> MATPDQKSPNVLLQNLCCRILGKSEADVAQQFQYAVRVIGSNFAPTVERDEFLVAEKIKKELTRQRREADAALFSELHRKLHSQGVLKNKWSILYLLLSLSEDPRKQPSKVSGYAALFAQALPRDAHSTPYYYARPQSLPLNYQERGAPSAQSAGSAGSSGVSSLGTYALNGPTPPPPPPALLPGQPLPAPGVGDGLRQQLGSRLAWTLTASQPSLPSTTSKAVPSSGSRGAARPRREGDAAAGAVEVTEAALVRDILYVFQGIDGKHVKMSNADNCYTVEGKANLSKSLRDTAVRLAELGWLHNKIRKYTDQRSLDRSFGLVGQSFCAALHQELREYYRLLSVLHSQLQLEDDQGVNLGLESSLTLRRLLVWTYDPKMRLKTLAALVDHCQGRKGGELASAVHAYTKTGDPYARSLVQHILSLVSHPVLSFLYRWIYDGELEDTYHEFFVASDPAVKADRLWHDKYALRKPMIPSFMTMDQCRKVLLIGKSINFLHQVCHDQT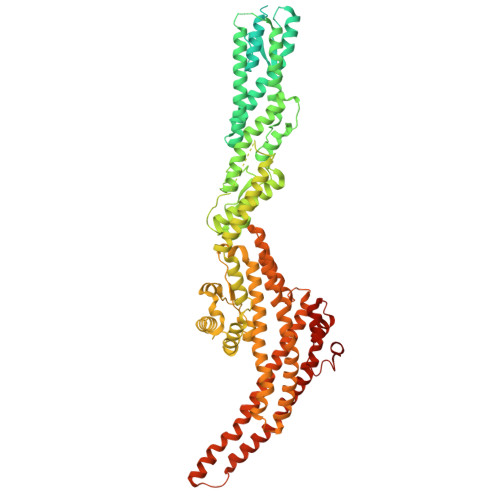PTTKMIAVTKSAESPQDAADLFTDLENAFQGKIDAAYFETSKYLLDVLNKKYSLLDHMQAMRRYLLLGQGDFIRHLMDLLKPELVRPATTLYQHNLTGILETAVRATNAQFDSPEILKRLDVRLLEVSPGDTGWDVFSLDYHVDGPIATVFTRECMSHYLRAFNFLWRAKRVEYILTDIRKGHMCNARLLRSMPEFSGVLHHCHILASEMVHFIHQMQYYVTFEVLECSWDELWNRVQRAQDLDHIIAAHEAFLGTVISRCLLDSDSRALLNQLRAVFDQIIELQNTQDAIYRAALEELQRRLQFEEKKKQREAEGQWGVSAAEEEQEKRRVQEFQESIPKMCSQLRILTHFYQGVVQQFLVSLTTSSDESLRFLSFRLDFNEHYRAREPRLRVSLGTRGRRSSHT>AAAASAPPAPADALPKGADSFFRTVISNMEKVYLSRNPTAKTILELVRSYDGDHICYDHFAFRTFGVDGYGIKSLAEFFTDFGYVPREELRFPAKKLRALWFSPPTNDGYTGTG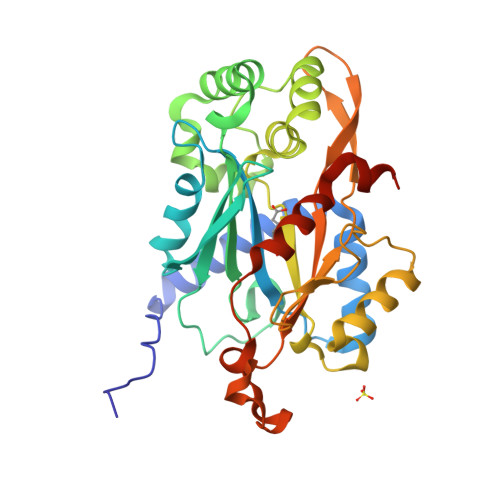VYGPLPRIFISELLVDELSPQSQDIIQKYIRTSGKGNKHATLASTSGELTWEKPIYSDFQVLSRESEYAAWTLVNGYALNHTTISTHRLISDIRSINKFNKFVEDNGFKLNSEGGILKVSPDGLLQQSSTVADSALFTFADGITESIPRSYIEFAERLVLPQFKDLPNDEVNEHHRRDGFEVGNADKIFESTSNDQLTRRSAHHHHHH[4x]The Agrobacterium tumefaciens genome contains two homologues of RNase D, Atu1151 (denoted At_RND, 30% similarity with full-length Ec_RND) and Atu4108 (denoted At_NrnC, 31% similarity with the N-terminal 184 residues of Ec_RND). At_RND contains an exonuclease domain and two HRDC domains, whereas At_NrnC contains a single DEDDy domain. At_NrnC forms an octameric hollow cylindrical structure, which allows dsDNA, ssDNA, and ssRNA to enter the central tunnel where the multiple active sites perform hydrolysis. This novel structural feature accounts for the high processivity of At_NrnC and its preference for longer dsDNA substrates despite the lack of HRDC domains.

The crystal structure of apo-At_NrnC was determined at 1.5 Å resolution and those of two forms of At_NrnC-Mn2+ were determined at 2.5 Å and 2.3 Å resolution. Metal binding was found to exert only a minor influence on the overall structure of At_NrnC. Based on the arrangement registered on the active pocket, we considered one of the metal-bound structures to represent an inactive state and the other an active state. In addition, nuclease assays indicated that Tyr153 is essential for At_NrnC function. Indeed, in the structure of the active state, Tyr153 was located at the typical catalytic site for DEDDy enzymes. In the active pocket, Asp27 and Asp86 coordinated one Mn2+, while Glu29 and Asp157 coordinated the other Mn2+. The distance between the two Mn2+ ions was 6.5 Å in the inactive state and 3.9 Å in the active state. According to the superposition, the two Mn2+ ions were located on two sides of the DNA backbone, which is similar to the case of Mg2+ and Zn2+ in the Klenow fragment structure.

>GPGSMAATIRYHEGDISAEDAARYKGAIAIDTETLGLVPRRDRLCVVQLSSGDGTADVIRIAAGQKQAPNLVHMLADPARQKIFHYGRFDIAVLFHTFGVTTTPVFCTKIASRLCRTYTDRHGLKDNLKEMLEVDISKAQQSSDWAAETLSPAQLEYAASDVLYLHALRDKLTARLIRDGRIEHADACFAFLPTRAKLDLLGWDETDIFAHS[2x]>[2x]GSMTNRTDDEYPEAPSDRTHVKRYHWLARYDQ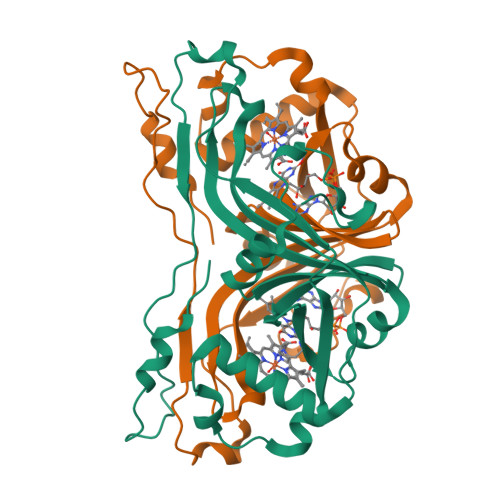ETVKAILDATPLAHVGCMMNGVPFVTPTFFWREGDRVYWHGSSAGRLFKALEHQDICLTVSLLDGLVIARSAYNFNCNFRSVMLLGRAELISDEAVKAEKLRNFVDGLIPGEWERLRPVHAKEIEATAVASLSIAEASCKVRTGPPLDDEEDYAFPSWAGVIPIRYQVLPPEPDPRNLPDVPMPEDILKFRLG>[16x]GAMAKETTPVALSFHDLHQLTRAAVERAQQLQVPVVVSIVDAHGTETVTWRMPDALLVSSELAPKKAWTAVAMKTATHELSDVVQPGAALYGLESHLQGKVVTFGGGYALWRDGILIGGLGISGGSVEQDMDIAQTAIAAINVGTHQ

Amongst its set of proteins, the pdu operon encodes PduO. This is an ATP:Cob(I)alamin adenosyltransferase (ACA) catalyzing the synthesis of adenosylcobalamin (AdoCbl; coenzyme B12). The Salmonella PduO is a two-domain protein, but only the N-terminal domain is necessary for the transferase activity. At the same time, the deletion mutant showed that the C-terminal domain and its heme binding are necessary for effective in vivo catabolism of 1,2-propanediol.

The PduOC:heme complex crystallized in the P21 space group with 2 octamers in the asymmetric unit (PDB acquisition code 5CX71). Each monomer has a three-layer, α-β-α folding that resembles the profilin fold. The octamer structure buries a large fraction of the monomers, leaving the two antiparallel α-helices exposed (right), but hiding the other three helices from the solvent. Across one interface, the β-sheets from monomers are hydrogen bonded, so as to form a large, regular 8-stranded sheet spanning pairs of dimers. Each octamer binds four heme molecules with each heme sitting in a pocket formed by the extended β-strand and an α-helix from each of two dimers. The heme iron is hexa-coordinated with bis-histidyl (bis-His) ligation by two histidines (H18) from adjacent monomers. The symmetry is such that pairs of corresponding residues from adjacent chains form the pocket (Phe14, His18, Thr21, Arg22, Val25, Val48, and Trp50). The eight heme groups in the asymmetric unit are highly exposed, with solvent accessible areas from 251 to 302 Å2. The exchange of His18 by Ala abolishes heme binding and this shifts the equilibrium from octamers to dimers. The bis-His heme coordination in PduOC is consistent with a possible role in electron transfer.pyridin-2-ol 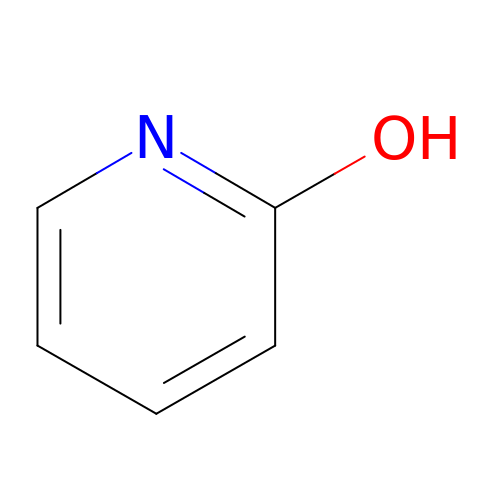| C5 H5 N O | UBQKCCHYAOITMY-UHFFFAOYSA-N In this work we investigate the use of a monosubstituted amino acid in the creation of a hydrocarbon constraint using Bcl-2/BH3 family PPIs as a model. This family of proteins play a pivotal role in the regulation of apoptosis, play a major role in cancer development/progression and represent key targets for anticancer drug-discovery The regulation of apoptosis exploits varying specificity and selectivity of pairwise interactions within the Bcl-2 family interactome. The canonical structural motif involves a BH3 domain from one Bcl-2 family member adopting a helical conformation and binding to a BH3 binding cleft of another partner. In this manuscript we report on the use of a novel α-alkenylglycine derived amino acid to synthesise hydrocarbon constrained BH3-family sequences (BIM and BID). Our biophysical and structural analyses illustrate that whilst the introduction of the constraint increases the population of the bioactive α-helical conformation of the peptide in solution, it does not enhance the inhibitory potency against pro-apoptotic Bcl-xL and Mcl-1 PPIs.

For a full comparison, we also synthesized the disubstituted amino acid and incorporated this, the monosubstituted amino acid and aminoisobutyric acid (Aib) at appropriate positions in the BID sequence (replacing 92Gln and 96Ser). To ascertain whether the constraint alters the recognition of the hot-spot residues within the peptide, BID-MM was co-crystallised with Mcl-1. When in complex with Mcl-1, the hydrocarbon constraint in BID-MM is positioned away from the protein surface, hence not contributing directly to binding. The double bond within the constraint is in a cis configuration, with no electron density to suggest that it exists in a trans configuration (ESI Fig. S11†). BID-MM binds analogously to BIM-WT in such a way that the constraint doesn't affect the positioning of the hot-spot residues. The salt bridge between the conserved BH3 aspartic acid and a conserved arginine in the BH1 domain of Mcl-1 is also retained. We then tested BID-MM and BID-DM against Mcl-1/FITC-NOXA-B in a FA based competition assay. In competition against this different Bcl-2/BH3 pairing, BID-MM was less potent, with an IC50 of 1.6 μM in comparison to 0.39 μM with BID-WT, whilst BID-DM was slightly better than BID-MM, with an IC50 of 0.8 μM. Crystal structures of Mcl-1/BID-MM and Bcl-xL/BIM-MM revealed that the constrained peptides adopt comparable binding conformations when compared to available structures with wild type sequences and/or peptides constrained with the α,α′-disubstituted alkenyl amino acids. Furthermore our structures confirm that the constraints point away from the BH3 binding cleft and do not introduce steric constraints or new non-covalent interactions with the anti-apoptotic partner.

> SELYRQSLEIISRYLREQATGAKDTKPMGRSGATSRKALETLRRVGDGVQRNHETAFQGMLRKLDIKNEDDVKSLSRVMIHVFSDGVTNWGRIVTLISFGAFVAKHLKTINQESCIEPLAESITDVLVRTKRDWLVKQRGWDGFVEFFHVEDLEGG;> XEDIIRNIARHLALVGDLLDRSIW>[6x]MKPEVEQELAHILLTELLAYQFASPVRWIETQDVFLKDFNTERVVEIGPSPTLAGMAQRTLKNKYESYDAALSLHREILCYSKDAKEIYYTPDPSELAAKEEPAKEEAPAPTPAASAPAPAAAAPAPVAAAAPAAAAAEIADEPVKASLLLHVLVAHKLKKSLDSIPMSKTIKDLVGGKSTVQNEILGDLGKEFGTTPEKPEETPLEELAETFQDTFSGALGKQSSSLLSRLISSKMPGGFTITVARKYLQTRWGLPSGRQDGVLLVALSNEPAARLGSEADAKAFLDSMAQKYASIVGVDLSSAASASGAAGAGAAAGAAMIDAGALEEITKDHKVLARQQLQVLARYLKMDLDNGERKFLKEKDTV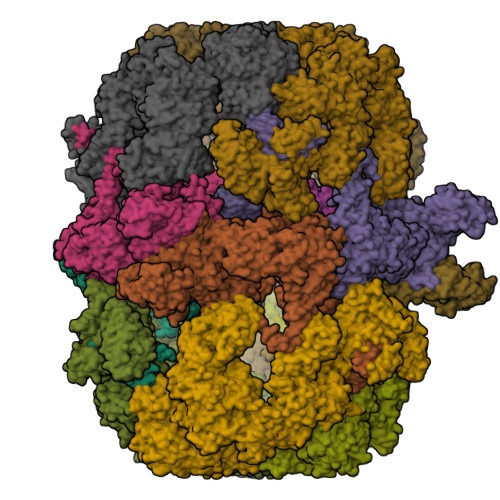AELQAQLDYLNAELGEFFVNGVATSFSRKKARTFDSSWNWAKQSLLSLYFEIIHGVLKNVDREVVSEAINIMNRSNDALIKFMEYHISNTDETKGENYQLVKTLGEQLIENCKQVLDVDPVYKDVAKPTGPKTAIDKNGNITYSEEPREKVRKLSQYVQEMALGGPITKESQPTIEEDLTRVYKAISAQADKQDISSSTRVEFEKLYSDLMKFLESSKEIDPSQTTQLAGMDVEDALDKDSTKEVASLPNKSTISKTVSSTIPRETIPFLHLRKKTPAGDWKYDRQLSSLFLDGLEKAAFNGVTFKDKYVLITGAGKGSIGAEVLQGLLQGGAKVVVTTSRFSKQVTDYYQSIYAKYGAKGSTLIVVPFNQGSKQDVEALIEFIYDTEKNGGLGWDLDAIIPFAAIPEQGIELEHIDSKSEFAHRIMLTNILRMMGCVKKQKSARGIETRPAQVILPMSPNHGTFGGDGMYSESKLSLETLFNRWHSESWANQLTVCGAIIGWTRGTGLMSANNIIAEGIEKMGVRTFSQKEMAFNLLGLLTPEVVELCQKSPVMADLNGGLQFVPELKEFTAKLRKELVETSEVRKAVSIETALEHKVVNGNSADAAYAQVEIQPRANIQLDFPELKPYKQVKQIAPAELEGLLDLERVIVVTGFAEVGPWGSARTRWEMEAFGEFSLEGCVEMAWIMGFISYHNGNLKGRPYTGWVDSKTKEPVDDKDVKAKYETSILEHSGIRLIEPELFNGYNPEKKEMIQEVIVEEDLEPFEASKETAEQFKHQHGDKVDIFEIPETGEYSVKLLKGATLYIPKALRFDRLVAGQIPTGWNAKTYGISDDIISQVDPITLFVLVSVVEAFIASGITDPYEMYKYVHVSEVGNCSGSGMGGVSALRGMFKDRFKDEPVQNDILQESFINTMSAWVNMLLISSSGPIKTPVGACATSVESVDIGVETILSGKARICIVGGYDDFQEEGSFEFGNMKATSNTLEEFEHGRTPAEMSRPATTTRNGFMEAQGAGIQIIMQADLALKMGVPIYGIVAMAATATDKIGRSVPAPGKGILTTAREHHSSVKYASPNLNMKYRKRQLVTREAQIKDWVENELEALKLEAEEIPSEDQNEFLLERTREIHNEAESQLRAAQQQWGNDFYKRDPRIAPLRGALATYGLTIDDLGVASFHGTSTKANDKNESATINEMMKHLGRSEGNPVIGVFQKFLTGHPKGAAGAWMMNGALQILNSGIIPGNRNADNVDKILEQFEYVLYPSKTLKTDGVRAVSITSFGFGQKGGQAIVVHPDYLYGAITEDRYNEYVAKVSAREKSAYKFFHNGMIYNKLFVSKEHAPYTDELEEDVYLDPLARVSKDKKSGSLTFNSKNIQSKDSYINANTIETAKMIENMTKEKVSNGGVGVDVELITSINVENDTFIERNFTPQEIEYCSAQPSVQSSFAGTWSAKEAVFKSLGVKSLGGGAALKDIEIVRVNKNAPAVELHGNAKKAAEEAGVTDVKVSISHDDLQAVAVAVSTKK;>[6x]STRPLTLSHGSLEHVLLVPTASFFIASQLQEQFNKILPEPTEGFAADDEPTTPAELVGKFLGYVSSLVEPSKVGQFDQVLNLCLTEFENCYLEGNDIHALAAKLLQENDTTLVKTKELIKNYITARIMAKRPFDKKSNSALFRAVGEGNAQLVAIFGGQGNTDDYFEELRDLYQTYHVLVGDLIKFSAETLSELIRTTLDAEKVFTQGLNILEWLENPSNTPDKDYLLSIPISCPLIGVIQLAHYVVTAKLLGFTPGELRSYLKGATGHSQGLVTAVAIAETDSWESFFVSVRKAITVLFFIGVRCYEAYPNTSLPPSILEDSLENNEGVPSPMLSISNLTQEQVQDYVNKTNSHLPAGKQVEISLVNGAKNLVVSGPPQSLYGLNLTLRKAKAPSGLDQSRIPFSERKLKFSNRFLPVASPFHSHLLVPASDLINKDLVKNNVSFNAKDIQIPVYDTFDGSDLRVLSGSISERIVDCIIRLPVKWETTTQFKATHILDFGPGGASGLGVLTHRNKDGTGVRVIVAGTLDINPDDDYGFKQEIFDVTSNGLKKNPNWLEEYHPKLIKNKSGKIFVETKFSKLIGRPPLLVPGMTPCTVSPDFVAATTNAGYTIELAGGGYFSAAGMTAAIDSVVSQIEKGSTFGINLIYVNPFMLQWGIPLIKELRSKGYPIQFLTIGAGVPSLEVASEYIETLGLKYLGLKPGSIDAISQVINIAKAHPNFPIALQWTGGRGGGHHSFEDAHTPMLQMYSKIRRHPNIMLIFGSGFGSADDTYPYLTGEWSTKFDYPPMPFDGFLFGSRVMIAKEVKTSPDAKKCIAACTGVPDDKWEQTYKKPTGGIVTVRSEMGEPIHKIATRGVMLWKEFDETIFNLPKNKLVPTLEAKRDYIISRLNADFQKPWFATVNGQARDLATMTYEEVAKRLVELMFIRSTNSWFDVTWRTFTGDFLRRVEERFTKSKTLSLIQSYSLLDKPDEAIEKVFNAYPAAREQFLNAQDIDHFLSMCQNPMQKPVPFVPVLDRRFEIFFKKDSLWQSEHLEAVVDQDVQRTCILHGPVAAQFTKVIDEPIKSIMDGIHDGHIKKLLHQYYGDDESKIPAVEYFGGESPVDVQSDSEDSAVFKATSSTDEESWFKALAGSEINWRHASFLCSFITQDKMFVSNPIRKVFKPSQGMVVEISNGNTSSKTVVTLSEPVQGELKPTVILKLLKENIIQMEMIENRTMDGKPVSLPLLYNFNPDNGFAPISEVMEDRNQRIKEMYWKLWIDEPFNLDFDPRDVIKGKDFEITAKEVYDFTHAVGNNCEDFVSRPDRTMLAPMDFAIVVGWRAIIKAIFPNTVDGDLLKLVHLSNGYKMIPGAKPLQVGDVVSTTAVIESVVNQPTGKIVDVVGTLSRNGKPVMEVTSSFFYRGNYTDFENTFQKTVEPVYQMHIKTSKDIAVLRSKEWFQLDDEDFDLLNKTLTFETETEVTFKNANIFSSVKCFGPIKVELPTKETVEIGIVDYEAGASHGNPVVDFLKRNGSTLEQKVNLENPIPIAVLDSYTPSTNEPYARVSGDLNPIHVSRHFASYANLPGTITHGMFSSASVRALIENWAADSVSSRVRGYTCQFVDMVLPNTALKTSIQHVGMINGRKLIKFETRNEDDVVVLTGEAEIEQPVTTFVFTGQGSQEQGMGMDLYKTSKAAQDVWNRADNHFKDTYGFSILDIVINNPVNLTIHFGGEKGKRIRENYSAMIFETIVDGKLKTEKIFKEINEHSTSYTFRSEKGLLSATQFTQPALTLMEKAAFEDLKSKGLIPADATFAGHSLGEYAALASLADVMSIESLVEVVFYRGMTMQVAVPRDELGRSNYGMIAINPGRVAASFSQEALQYVVERVGKRTGWLVEIVNYNVENQQYVAAGDLRALDTVTNVLNFIKLQKIDIIELQKSLSLEEVEGHLFEIIDEASKKSAVKPRPLKLERGFACIPLVGISVPFHSTYLMNGVKPFKSFLKKNIIKENVKVARLAGKYIPNLTAKPFQVTKEYFQDVYDLTGSEPIKEIIDNWEKYEQ> MHGAEHLLEIFYLLLAAQVCAFIFKRLNQPVVIGEVLAGVLVGPALLGLVHEGEILEFLAELGAVFLLFMVGLETRLKDILAVGKEAFLVAVLGVALPFLGGYLYGLEIGFETLPALFLGTALVATSVGITARVLQELGVLSRPYSRIILGAAVIDDVLGLIVLACVNGVAETGQVEVGAITRLIVLSVVFVGLAVFLSTLIARLPLERLPVGSPLGFALALGVGMAALAASIGLAPIVGAFLGGMLLSEVREKYRLEEPIFAIESFLAP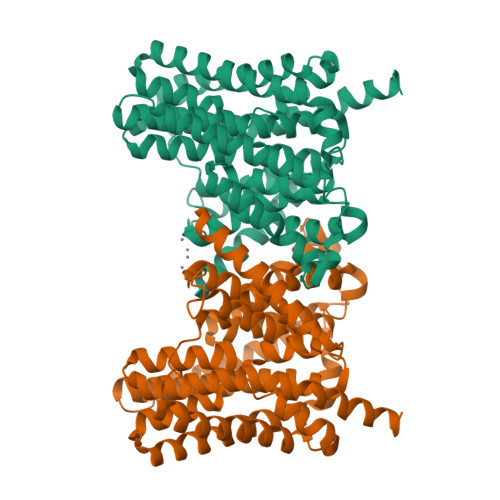IFFAMVGVRLELSALASPVVLVAGTVVTVIAILGKVLGGFLGALTQGVRSALTVGCGMAPRGEVGLIVAALGLKAGAVNEEEYAIVLFMVVFTTLFAPFALKPLIAWTERERAAKEGSENLYFQ>[2x]MALSKQYIPDDMELIFHMDGNVNGHYFTIVATGKAKPYEGKQNLKATVTKGAPLPFSTDILSTVMHYGNRCIVHYPPGIPDYFKQSFPEGYSWERTFAFEDGGFCTVSADIKLKDNCF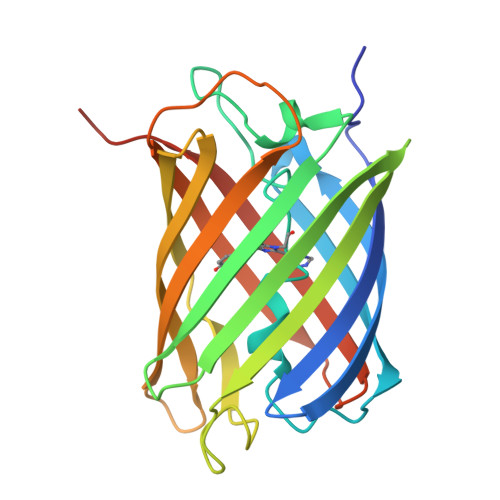IHTSMFHGTNFPADGPVMQRKTIQWEKSIEKMTVSDGIVKGDITMFLLLEGGGKYRCQFHTSYKAKKVVEMPQSHYVEHSIERTNDDGTQFELNEHAVARLNEILEHHHHHH>GAMDPREVILCKDQDGKIGLRLKSIDNGIFVQLVQANSPASLVGLRFGDQVLQINGENCAGWSSDKAHKVLKQAFGEKITMTIRDRPFERTITMHKDSTGHVGFIFKNGKITSIVKDSSAAR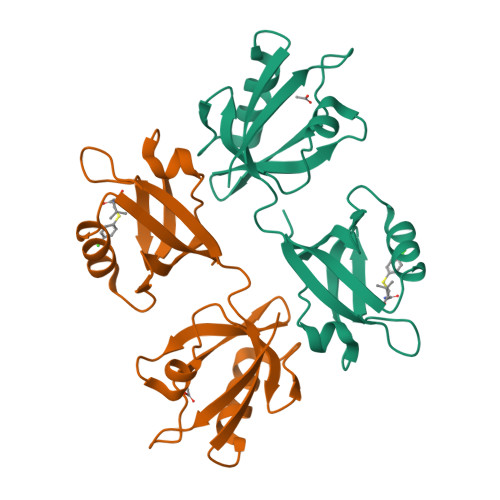NGLLTEHNICEINGQNVIGLKDSQIADILSTSGTVVTITIMPAF[4x]> GPAMENILDLWNQALAQIEKKLSKPSFETWMKSTKAHSLQGDTLTITAPNEFARDWLESRYLHLIADTIYELTGEELSIK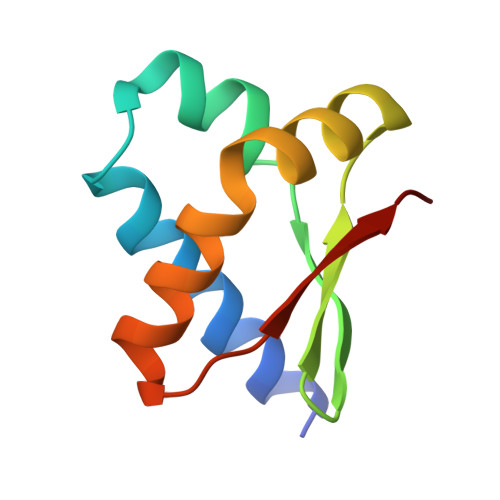FVIPQ>GTGYTVGDFMTPRQNLHVVKPSTSVDDALELLVEKKVTGLPVIDDNWTLVGVVSDYDLLALDSISGRSQNDTNLFPDVDSTWKTFNELQKLISKTYGKVVGDLMTPSPLVVRDSTNLEDAARLLLETKFRRLPVVDADGKLIGILTRGNVVRAALQIKRN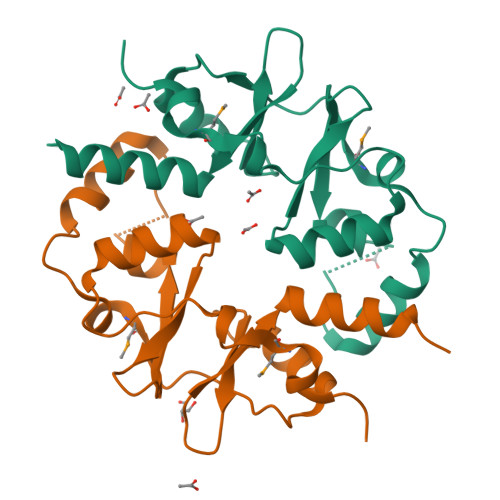ADSISGRSQNDTNLFPDVDS[2x]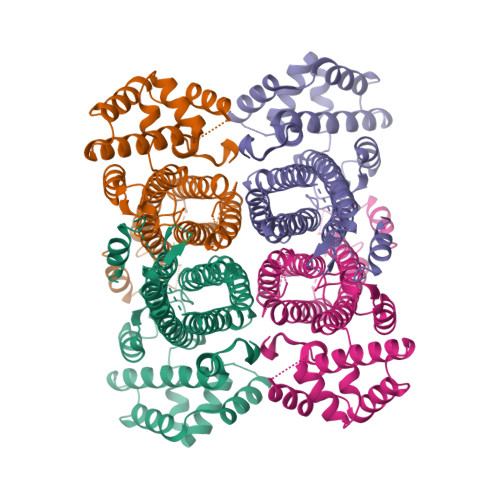>MGSSHHHHHHSSGENLYFQGHMIARYQTPEMARLWSEESRYRMWARVEAYALEAWEALGEVPKGLSARLLAKLEEKPLDGAFARRVAELEAVTRHDLVAFTRALAEWTGDEEVGRYLHLGLTSSDIVDTAQNALLVEALGLVLEELKGVEEALKALALRHKHTPAIARTHGVHAEPTSFGLRFLSFLAAFQRDEERLKRARETIGVAMLSGSVGNYAHVPPEVEAHVASRLGLRPEPLSTQVVPRDRHAEVMAALAILGGNIERVAVELRHLQRTEVLEAQEPFHEGQTGSSSMPHKKNPVGLENLTGVARLLRGYLFPALEDIALWHERDISHSSVERVILPDATTLAHYALRRLKGILEGLEVFEENLARNLDLTRGLVYSQQVLNALIARGLSRNKAYALVQRNALRSWKEGKSFLELLEADPENPLKGKELRALFDPKPFLRHVDAIYARFGL[2x]>[4x]GPSLTQLCNRRKLWADFRAAFARAKRLRQPLSCISIDIDNFKLINDQFGHDKGDEVLCFLAKLFQSVISDHHFCGRVGGEEFIIV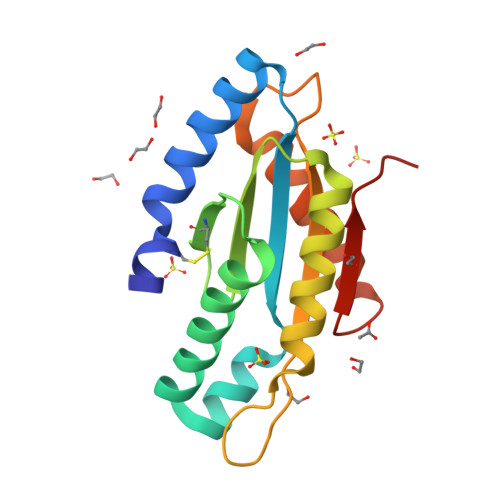LENTHVETAFHLAEQIRQRFAEHPFFEQNEHIYLCAGVSSLHHGDHDIADIYRRSDQALYKAKRNGRNRCCIYRQSTE> ASYVVNNENIDKDGRQAY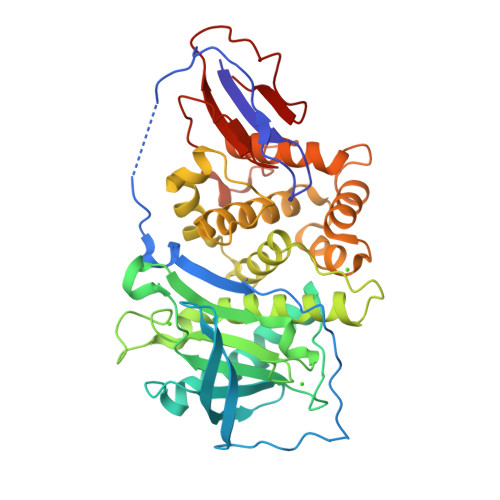TGSYNRAALKQQTVKQMGPQNREAFKEDKLFKAPKNKQPIRKSENRSQNGGKQYSLNDQRTFTTIDNRTNQDEQTTATLKYDGKKAQVWVADQYITDKQAQNIGREFDERIDPLIENNFGEPSDVDNNGKVNILVYDIKDNYDQTGTYIGGYFHPRDLYNVRGSNHSEIFYMDTYPSMGTDRQHLNESQIYSTLAHQYQHMVNANENLFKEQSQEEMDPWLNEALSMASEQMYLNAPLNSRIDYYNNSKSIAYGHSLIRWDEQGDTLSNFSLSYLFIEYLKKQSDNGEQVFKELINDPGDTNTALQNAIHEHVDPNLSLSKFMTNFRIALVKKENSGPYGFKGDADFNNVHPQPISQIPETLAPQGSVLFQTNQDFNVPNDKDEDISYNKVN D-alanyl-N-[(2S,6R)-6-amino-6-carboxy-1-{[(1R)-1-carboxyethyl]amino}-1-oxohexan-2-yl]-D-glutamine | C18 H31 N5 O9 | 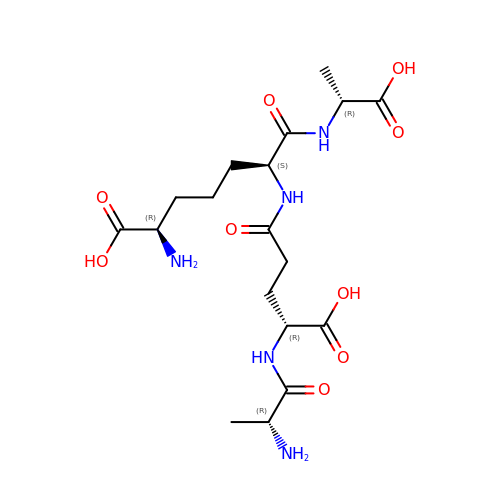VFGFFQOPKZHQLZ-PZWNZHSQSA-N>SDVDLSKYITTIAGVMTLSQVKGFVRKNGVNEAKIDEIKNDNVQDTAEQKVQLLRNWHQLHGKKEAYDTLIKDLKKANLCTLAEKIQTIILKDITS[7x];>APGEEDLCAAFNVICDNVGKDWRRLARQLKVSDTKIDSIEDRYPRNLTERVRESL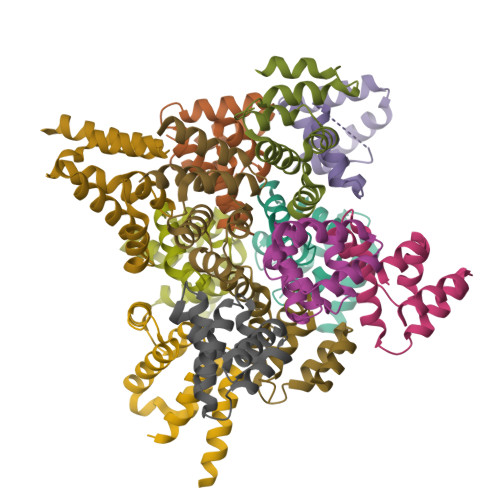RIWKNTEKENATVAHLVGALRSCQMNLVADLVQEVQQARDLQNRSG[5x]> DITVYNGQHKEAAQAVADAFTRATGIKVKLNCAKGDQLAGQIKEEGSRSPADVFYSEQIPALATLSAANLLEPLPASTINETRGKGVPVAAKKDWVALSGRSRVVVYDTRKLSEKDLEKSVLNYATPKWKNRIGYVPTSGAFLEQIVAIVKLKGEAAALKWLKGLKEYGKPYAKNSVALQAVENGEIDAALINNYYWHAFAREKGVQNVHTRLNFVRH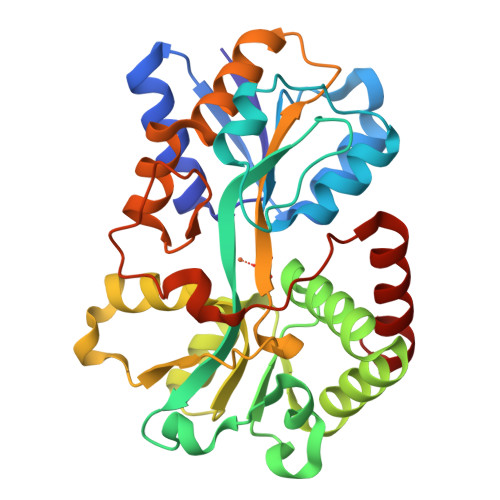RDPGALVTYSGAAVLKSSQNKDEAKKFVAFLAGKEGQRALTAVRAEYPLNPHVVSTFNLEPIAKLEAPQVSATTVSEKEHATRLLEQAGMK>[8x]MSSYSNKDVQRGDASMHHYQWAKTPPMGWNSWDCYGASVTEDEVKGNAEYMAKYLKPFGWEYVVVDIQWYEPGANSSIYRPFVPLEMDEYSRLMPAVNRFPSAKGGKGFKPLADYIHNLGLKFGIHIMRGIPRQAVH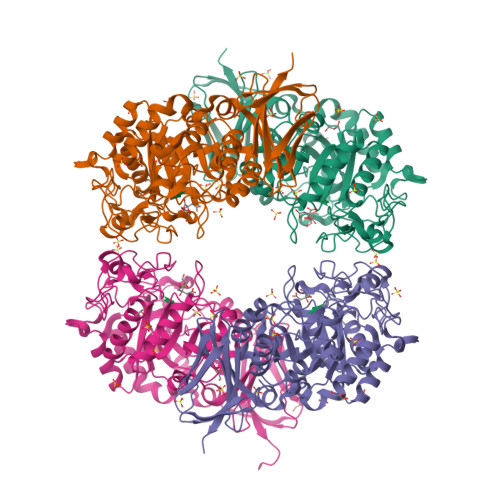QNTPILGTNVGARDIADTNSICPWNTDMYGVDHRKEGAQAYYDSLFQLYAQWGVDFVKVADIVASKLYGTHTEEIKMIRKAIDRCGRPIVLSLSPGPAPLDHATLFVENANMWRMTDDFWDRWELLYDMFEQCYKWCKLVGLGHWPDADMLPLGHIGIRSVDGGGTDRMTRFTKDEQRTMMTLWIIFRSPLMFGGELRDNDEWTLSLLTNEEVLHVHQNGYGARQVYRENDHVVWTSQDAEGNQFVAMFNISEKRSVVSVSLKDLGCMEPMKARDLWAKEDLGLVKHQLAFELGPHQSILVKLSPAVGKGL> GPH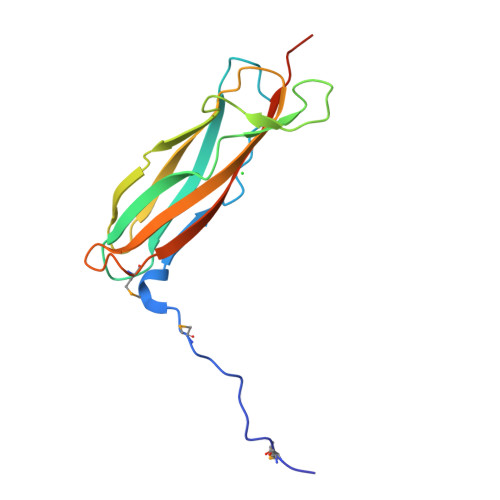MSVSHLVKPMTKPPSTKVEIRNKSITFPTTEPGETSESCLELENHGTTDVKWHLSSLAPPYVKGVDESGDVFRATYAAFRCSPISGLLESHGIQKVSITFLPRGRGDYAQFWDVECHPLKEPHMKHTLRFQLSGQSIEAENEPENACL2-azanyl-6-[(1~{S},7~{S})-2,2-bis(fluoranyl)-7-oxidanyl-cycloheptyl]-4-methoxy-7~{H}-pyrrolo[3,4-d]pyrimidin-5-one | C14 H18 F2 N4 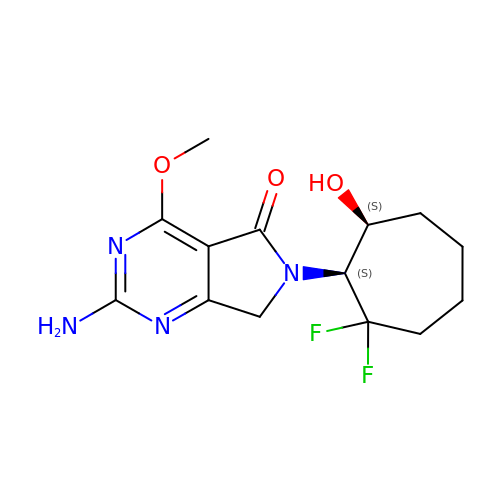O3 | VWSRMVWRUFUXMB-WPRPVWTQSA-N>[8x]HHHHHHENLYFQGENSDDYDLMYVNLDNEIDNGLHPTEDPTPCACGQEHSEWDKLFIMLENSQMRERMLLQATDDVLRGELQRLREELGRLAESLARPCAPGAPAEARLTSALDELLQATRDAGRRLARMEGAEAQRPEEAGRALAAVLEELRQTRA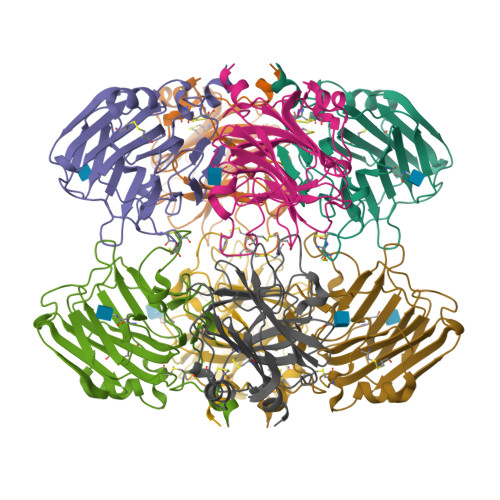DLHAVQGWAARSWLPAGCETAILFPMRSKKIFGSVHPVRPMRLESFSACIWVKATDVLNKTILFSYGTKRNPYEIQLYLSYQSIVFVVGGEENKLVAEAMVSLGRWTHLCGTWNSEEGLTSLWVNGELAATTVEMATGHIVPEGGILQIGQEKNGCCVGGGFDETLAFSGRLTGFNIWDSVLSNEEIRETGGAESCHIRGNIVGWGVTEIQPHGGAQYVS> IESIIKTATDTVKSEINAELGVVPSLNAVETGATSNTEPEEAIQTRTVINQHGVSETLVENFLSRAALVSKRSFEYKDHTSSTARADKNFFKWTINTRSFVQLRRKLELFTYLRFDAEITILTTVAVNGSGNNTYVGLPDLTLQAMFVPTGALTPEKQDSFHWQSGSNASVFFKISDPPARITIPFMCINSAYSVFYDGFAGFEKNGLYGINPADTIGNLCVRIVNEHQPVGFTVTVRVYMKPKHIKAWAPRPPRTLPYMSIANANYKGKERAPNALSAIIGNRDSVKTMPHNIVN;> SDRVLQLKLGNSAIVTQEAANYCCAYGEWPNYLPDHEAVAIDKPTQPETATDRFYTLKSVKWETGSTGWWWKLPDALNNIGMFGQNVQHHYLYRSGFLIHVQCNATKFHQGALLVVAIPEHQRGAHNTNTSPGFDDIMKGEEGGTFNHPYVLDDGTSLACATIFPHQWINLRTNNSATIVLPWMNAAPMDFPLRHNQWTLAIIPVVPLGTRTTSSMVPITVSIAPMCCEFNGLRHAIT;> GVPTYLLPGSGQFLTTDDHSSAPALPCFNPTPEMHIPGQVRNMLEVVQVESMMEINNTESAVGMERLKVDISALTDVDQLLFNIPL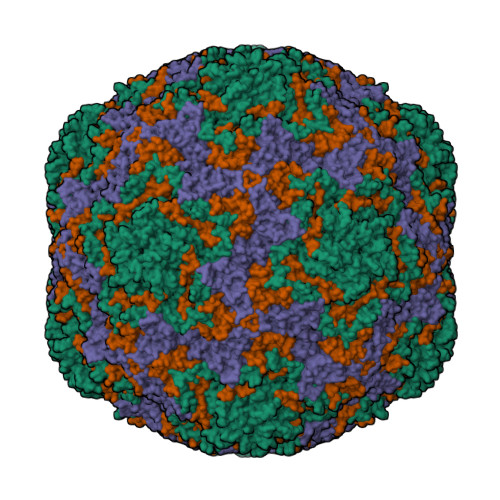DIQLDGPLRNTLVGNISRYYTHWSGSLEMTFMFCGSFMAAGKLILCYTPPGGSCPTTRETAMLGTHIVWDFGLQSSVTLIIPWISGSHYRMFNNDAKSTNANVGYVTCFMQTNLIVPSESSDTCSLIGFIAAKDDFSLRLMRDSPDIGQLDHLHAAEAAYQ;> GAQVTRQQTGTHENANIATNGSHITYNQINFYKDSYAASASKQDFSQDPSKFTEPVVEGLKAGAPVLK> MAKKTSSKGKPPGPFAWPLIGNAAAVGQAAHLSFARLARRYGDVFQIRLGSCPIVVLNGERAIHQALVQQGSAFADRPSFASFRVVSGGRSMAFGHYSEHWKVQRRAAHSMMRNFFTRQPRSRQVLEGHVLSEARELVALLVRGSADGAFL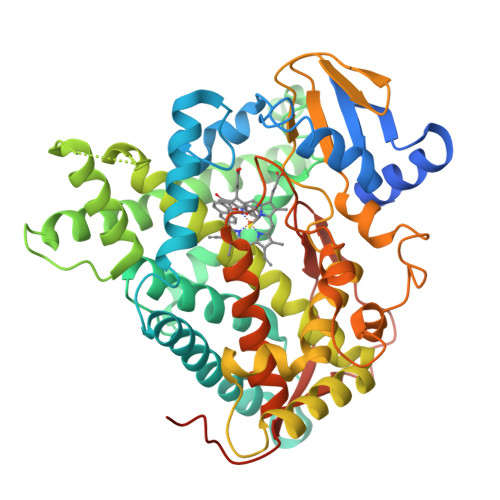DPRPLTVVAVANVMSAVCFGCRYSHDDPEFRELLSHNEEFGRTVGAGSLVDVMPWLQYFPNPVRTVFREFEQLNRNFSNFILDKFLRHCESLRPGAAPRDMMDAFILSAEKKAAGDSHGGGARLDLENVPATITDIFGASQDTLSTALQWLLLLFTRYPDVQTRVQAELDQVVGRDRLPCMGDQPNLPYVLAFLYEAMRFSSFVPVTIPHATTANTSVLGYHIPKDTVVFVNQWSVNHDPLKWPNPENFDPARFLDKDGLINKDLTSRVMIFSVGKRRCIGEELSKMQLFLFISILAHQCDFRANPNEPAKMNFSYGLTIKPKSFKVNVTLRESMELLDSAVQNLQAKETCQHHHH> GHMKRLAVFASGSGTNFQAIVDAAKRGDLPARVALLVCDRPGAKVIERAARENVPAFVFSPKDYPSKAAFESEILRELKGRQIDWIA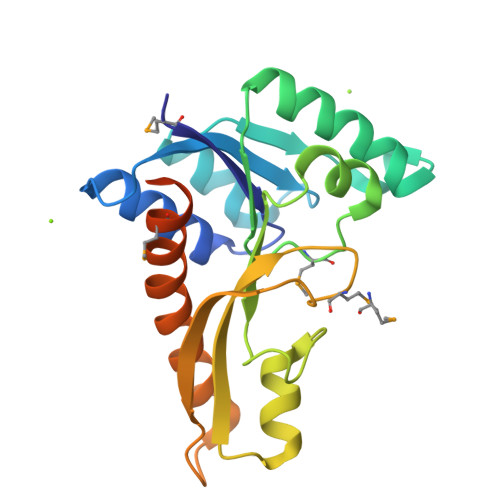LAGYMRLIGPTLLSAYEGKIVNIHPSLLPAFPGKDAIGQAYRAGVSETGVTVHYVDEGMDTGPVIAQRVVPIVPGEPIEALEERIHQVEHELYPTVLRMLLGEKEQQEERIENDGSETSIDQRVQ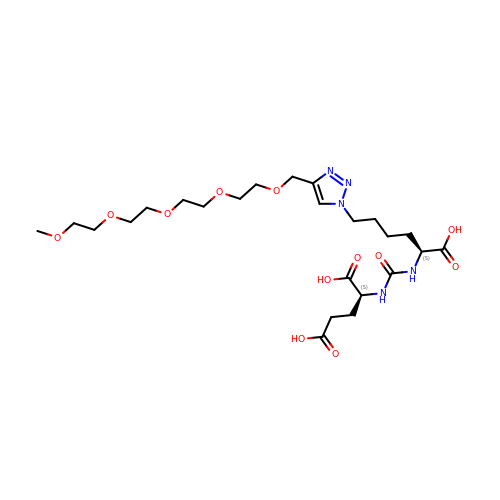N-({(1S)-1-CARBOXY-5-[4-(2,5,8,11,14-PENTAOXAPENTADEC-1-YL)-1H-1,2,3-TRIAZOL-1-YL]PENTYL}CARBAMOYL)-L-GLUTAMIC ACID | C24 H41 N5 O12 | USQOBCXXBZGYAH-PMACEKPBSA-N>MAQSSNSTHEPLEVLKEETVNRHRAIVSVMEELEAVDWYDQRVDASTDPELTAILAHNRDEEKEHAAMTLEWLRRNDAKWAEHLRTYLFTEGPITAANSSSVDKLAAALEHHHHHH[30x]

Our study reports on a new class of ferritin-like proteins (EncFtn), which are associated with bacterial encapsulin nanocompartments (Enc). By studying the EncFtn from R. rubrum we demonstrate that iron binding results in assembly of EncFtn decamers, which display a unique annular architecture. Biochemical assays show that EncFtn is active as a ferroxidase enzyme. While EncFtn does not store iron itself, its association with the encapsulin nanocage suggests that mineralization occurs within the cavity of the encapsulin shell (McHugh et al., 2014).

The crystal structure of a truncated hexahistidine-tagged variant of the EncFtn protein (EncFtnsH) shows that it forms a decameric structure with an annular ‘ring-doughnut’ topology, which is distinct from the four-helical bundles of the 24meric ferritins and dodecahedral DPS proteins. We identify a symmetrical iron bound ferroxidase center (FOC) formed between subunits in the decamer and additional metal-binding sites close to the center of the ring and on the outer surface. Despite a radically different quaternary structure to the classical ferritins, the four-helical bundle scaffold and FOC of EncFtnsH are strikingly similar to ferritin. A structural alignment of the FOC of EncFtn with the classical ferritin PmFtn shows that the central ring of EncFtn corresponds to the external surface of ferritin, while the outer circumference of EncFtn is congruent with the inner mineralization surface of ferritin. This overlay highlights the fact that the ferroxidase center of EncFtn faces in the opposite direction relative to the classical ferritins and is essentially inside out regarding iron storage space (boxed region). Furthermore, the position of the calcium ion coordinated by Glu31 and Glu34 seen in the EncFtnsH structure suggests an entry site to channel metal ions into the FOC; we propose that this site binds hydrated iron ions in vivo and acts as a selectivity filter and gate for the FOC. The constellation of charged residues on the outer circumference of EncFtn (His57, Glu61 and Glu64) could function in the same way as the residues lining the mineralization surface within the classical ferritin nanocage, and given their proximity to the FOC these sites may be the exit portal and mineralization site. The five metal-binding sites on the interior of the ring (Glu31/34-sites) may select for the Fe2+ ion and direct it towards their cognate FOCs. We propose that the oxidation of Fe2+ to Fe3+ occurs within the FOC according to the model postulated by in which the FOC acts as a substrate site through which iron passes and is released on to weakly coordinating sites at the outer circumference of the protein (His57, Glu61 and Glu64), where it is able to form ferrihydrite minerals which can be safely deposited within the lumen of the encapsulin nanocompartment.> GQSYEELIEKSYDFVDKGDLVSAEESLKAAMRK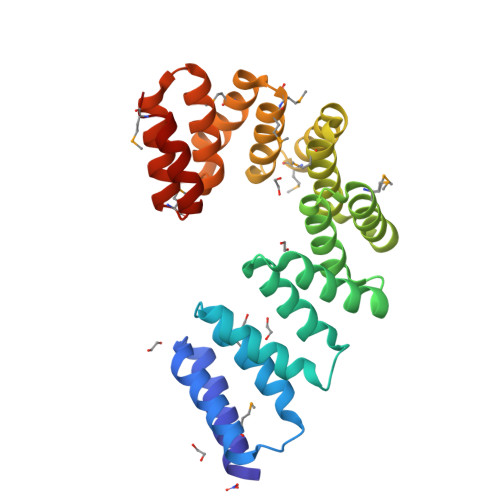EPANPLNYALLTNLGTIQRRQGKLQEALISYTSALSGHTKNITILENRASLYTELGETEKALNDYNTLLIENPEHQEALYCRGLLYIQLQNYMWAEQDFDKILEVNEKSVRARLGHAILEKMRGNYDESERIFNYLISEMPRDWILYEGRADLYFMMGKNARAMADIEKVFTESEPTANLYVLRGKIKLAQYEKERAALDFKKAESMGYNKEVIKELLKLTMNN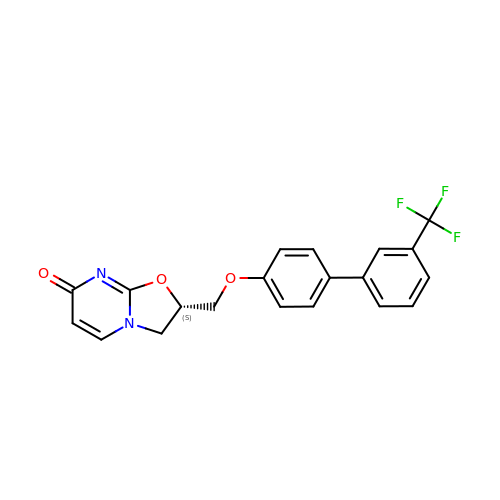(2S)-2-({[3'-(trifluoromethyl)[1,1'-biphenyl]-4-yl]oxy}methyl)-2,3-dihydro-7H-[1,3]oxazolo[3,2-a]pyrimidin-7-one | C20 H15 F3 N2 O3 | AYYWUDDPGRDIQB-KRWDZBQOSA-N>VSFNYTRFKDDGSLIFQGDAKIWTDGRLAMPTDPLVNRTTSHALYATPVPIWDSATGNVASFITSFSFIVSNVQRYPPTDGVVFFLAPWGTEIPPNSQGGYLGITDSSNSQNQFVAVEFDSHPNVWDPKSLRSSHIGIDVNSIMSLKAVNWNRVS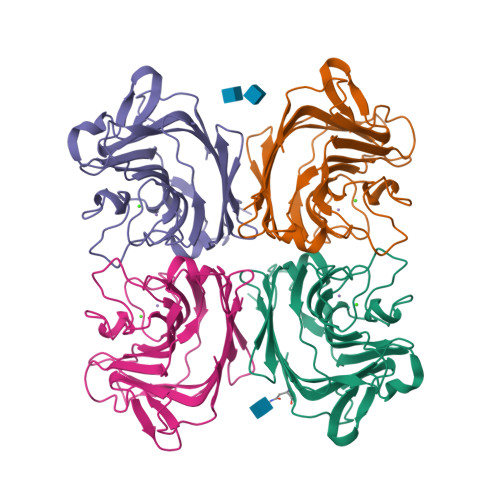GSLEKATIIYDSDTKILTVVMTHQNGQITTISQEIDLKTVLPEKVSVGFSATTWNPERERHDIYSWSFTSTLKEPEEQA[4x]5'-O-[(L-HISTIDYLAMINO)SULFONYL]ADENOSINE | C16 H21 N9 O7 S | 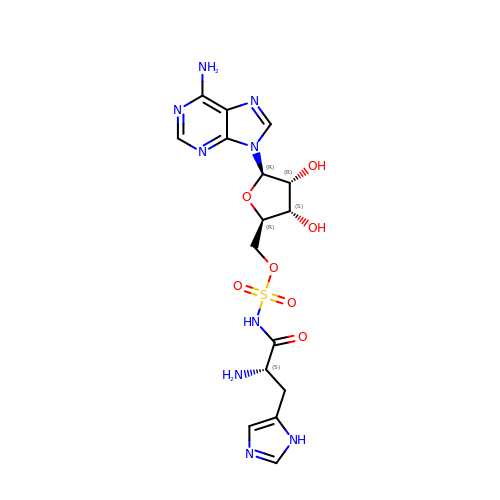WRXPXUSZYDNAQP-LEJQEAHTSA-N> 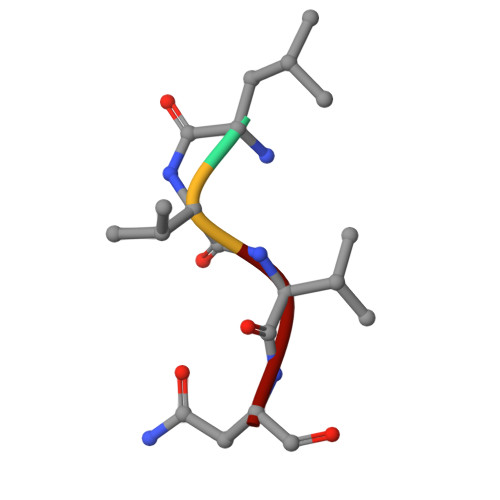LVVN> GF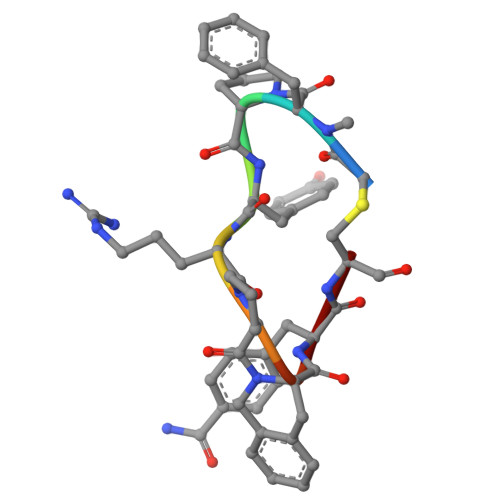PYRPXFC>[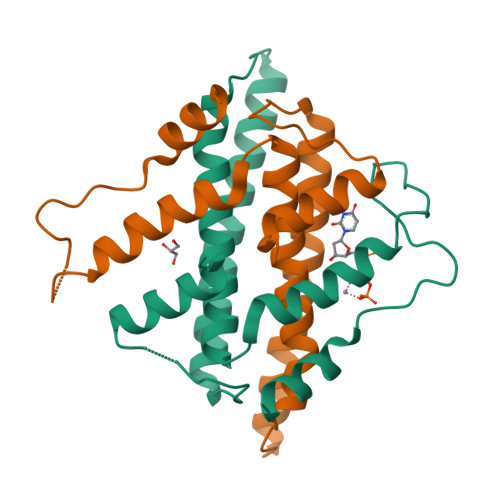2x]PPTNAERLHEFHRAIGAATPERPTPPPPELLRLRQTLLDAESAEVRAEIDHLLARQAAGEALSAGDLAPLAHELADLLYVTYGALDQLGIDADAVFAEVHRANLSKASGPRRADGKQLKPEGWRPADVRGVIERLQHA> GHKHSESVLQQFYNRLPVRKRFLKAIRKGTLIWDKGQVKIPPI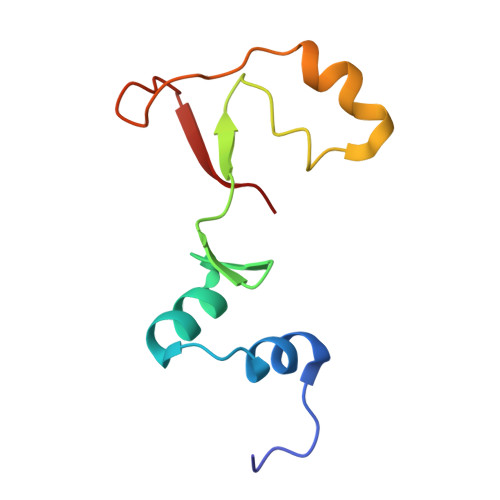AMQGYGLPNKLVLPHQKEFNNKLPKFKGKINQLKATRIWFQD> PCIEVVPNITYQCMDQKLSKVPDDIPSSTKNIDLSFNPLKILKSYSFSNFSELQWLDLSRCEIETIEDKAWHGLHHLSNLILTGNPIQSFSPGSFSGLTSLENLVAVETKLASLESFPIGQLITLKKLNVAHNFIHSCKLPAYFSNLTNLVHVDLSYNYIQTITVNDLQFLRENPQVNLSLDMSLNPIDFIQDQA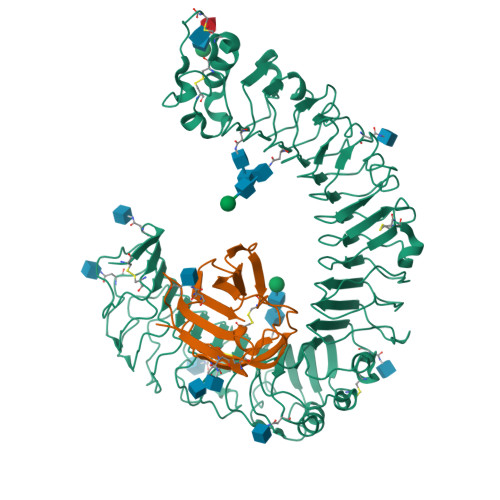FQGIKLHELTLRGNFNSSNIMKTCLQNLAGLHVHRLILGEFKDERNLEIFEPSIMEGLCDVTIDEFRLTYTNDFSDDIVKFHCLANVSAMSLAGVSIKYLEDVPKHFKWQSLSIIRCQLKQFPTLDLPFLKSLTLTMNKGSISFKKVALPSLSYLDLSRNALSFSGCCSYSDLGTNSLRHLDLSFNGAIIMSANFMGLEELQHLDFQHSTLKRVTEFSAFLSLEKLLYLDISYTNTKIDFDGIFLGLTSLNTLKMAGNSFKDNTLSNVFANTTNLTFLDLSKCQLEQISWGVFDTLHRLQLLNMSHNNLLFLDSSHYNQLYSLSTLDCSFNRIETSKGILQHFPKSLAFFNLTNNSVACICEHQKFLQWVKEQKQFLVNVEQMTCATPVEMNTSLVLDFNNSTC;> QQWFCNSSDAIISYSYCDHLKFPISISSEPCIRLRGTNGFVHVEFIPRGNLKYLYFNLFISVNSIELPKRKEVLCHGHDDDYSFCRALKGETVNTSIPFSFEGILFPKGHYRCVAEAIAGDTEEKLFCLNFTIIH[(3S)-3-{[8-(1-ethyl-5-methyl-1H-pyrazol-4-yl)-9-methyl-9H-purin-6-yl]oxy}pyrrolidin-1-yl](oxan-4-yl)methanone 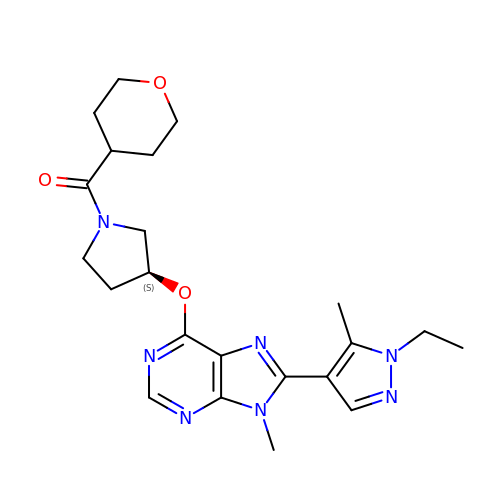| C22 H29 N7 O3 | FHKPLLOSJHHKNU-INIZCTEOSA-N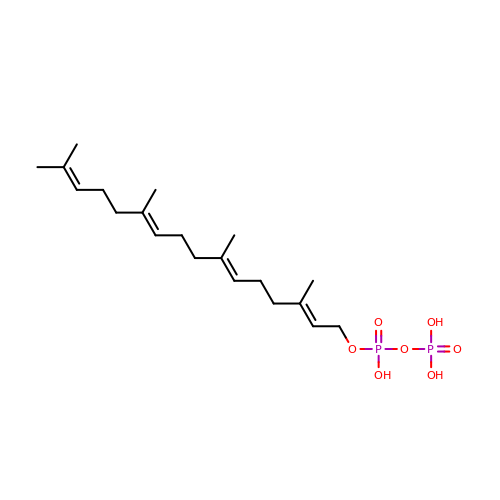NerylNeryl pyrophosphate | C20 H36 O7 P2 | OINNEUNVOZHBOX-UHFFFAOYSA-N Arginyl-tRNA-protein transferase 1 (ATE1) is a 58 kDa aminoacyl transferase that is conserved among nearly all eukaryotes. With the aid of a transfer RNA (tRNA) cofactor, ATE1 covalently adds arginine (arginylation) to its protein substrates to promote their degradation. The reaction requires arginyl-tRNAArg as the arginine donor, and ATE1 catalyzes the specific transfer of arginine to the first residue (Asp or Glu) of substrates. Here, we report two structures of ATE1 from Saccharomyces cerevisiae (scATE1) in apo form and in complex with tRNAArg.

We first determined the structure of full-length scATE1 using single-particle cryo-electron microscopy (cryoEM) to an average resolution of 3.2 Å. The structure of scATE1 displays an overall new fold with a compact conformation consisting of three domains, including a highly conserved GCN5-related N-acetyltransferases (GNAT) fold, a putative polypeptide substrate binding domain, and a unique variable domain. ScATE1 folds into a compact and globular conformation consisting of 18 well-defined β-strands along with 15 long and 9 short α-helices. DALI analysis for the rest of the structure returned no hits with a Z-score (typical range 2~60) above 4, indicating a new fold that is not represented in the PDB. Within this new fold, the N- and C- termini of scATE1 coalesce, forming a mixed β-sheet (β1-β18-β16-β17 and β2-β3-β5-β4) facing the GNAT domain. Notably, the electrostatic surface potential of the scATE1 defines a large positively charged surface area on the GNAT domain that could interact with negatively charged nucleic acid. Inspection of the cryoEM map with the modeled structure revealed density within the substrate binding domain that cannot be solely accounted for by protein sidechains. This density localizes to a highly conserved cystine cluster, comprised of C20, C23, C94 and C95, and is indicative of metal coordination. The melting temperature of scATE1 (46 °C) decreased with increasing concentrations of EDTA, suggesting that divalent metal ions are required to stabilize ATE1. Consistently, supplementing additional zinc ions further stabilized scATE1, as evidenced by an 8 °C shift in the thermal melting curve.

> MSDRFVIWAPSMHNEPAAKCGYCHGNKGGNMDQLFALDSWAHRYMNKMDVVKIENCTIGSFVEHMDVATYDRMCNMGFRRSGKFLYKVDPLRNCCRLYTIRTAPQELNMTKELKKCISRFATRITSEDYCPAAVASSDFVGKIVNAEMNSKTFYTRFEPALYSEEKYHLFVKYQEKVHQDYNNSPKSFKRFLCDTPFGPEAVLGTQESWEQLNNWQRMKPGEKLKHMGPVHECYYYEGKLIAITVSDILPSGISSVYFIWDPDYSKWSLGKLSALRDLAIIQRTNLQYYYLGYYIEDCPKMNYKANYGAEVLDVCHSKYIPLKPIQDMISRGKLFVIGEEETKVTKELYLVDSETGRGEGFPTDNVVKYKNIAEEIYGVGGCAFKSANESALELKELYGIPYEEEDLDTIYHLKEHNGHAPNGIPNVVPGLLPLWELLDIMQSGKITDLEGRLFLFEIETEGIRPLINFYSEPPNVKKRICDVIRLFGFETCMKAVILYSEQM> MEEASSISRYLYTFIVLFIIWLFLTASLDPQELTIGALFSAIAALFTYEIFTTRGLANLHPKRVLYFIAYIPYFLWAMIMANLDVAYRVLHPKRPINPGIVECKTTLTNNVGKMALANSITLTPGTITLDVDGDKYFIHWIDVKDSSVEGASE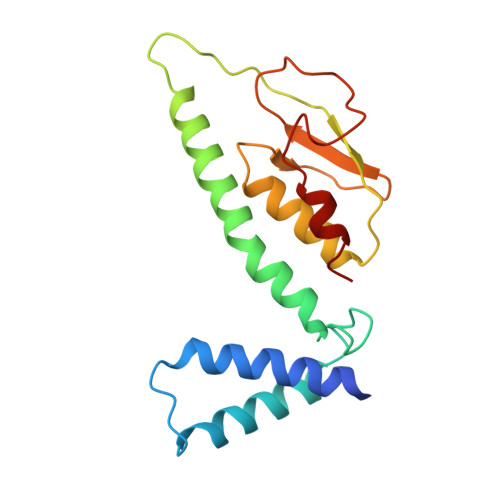HITKPFEKFLRVIFE> SLSQLSSQ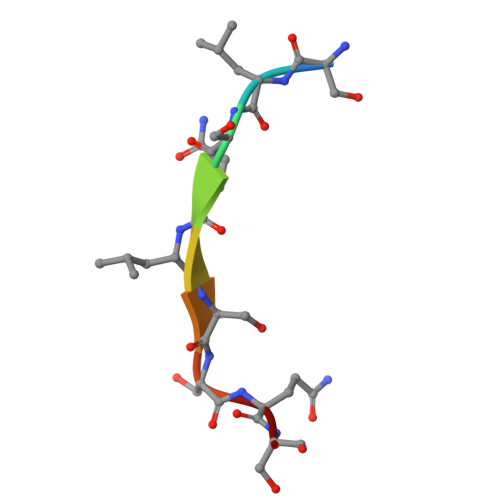S> MSLAIDLEVKQDVLIVRLSGELDHHTAEELREQVTDVLENRAIRHIVLNLGQLTFMDSSGLGVILGRYKQIKNVGGQMVVCAVSPAVK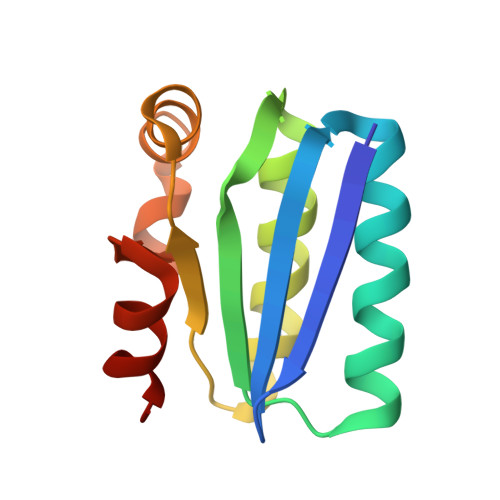RLFDMSGLFKIIRVEADEQFALQALGVA>MSGDNFLKAFAALEALAALPASAKELQLELIKQFMAEAMKIGNKEGLLLLAERLEALKPKVSPEIAVLVEKAAEMLKLLAKA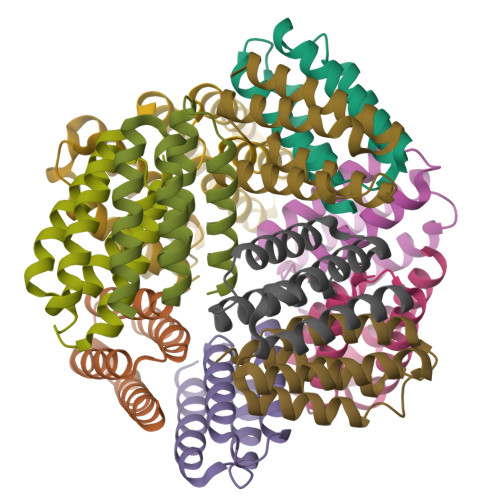L[24x]> PVFENNNQRYYESLPFKQLKELKIACSQYGPTAPFTIAMIENLGTQALPPNDWKQTARACLSGGDYLLWKSEFFEQCARIADVNRQQGIQTSYEMLIGEGPYQATDTQLNFLPGAYAQISNAARQAWKRL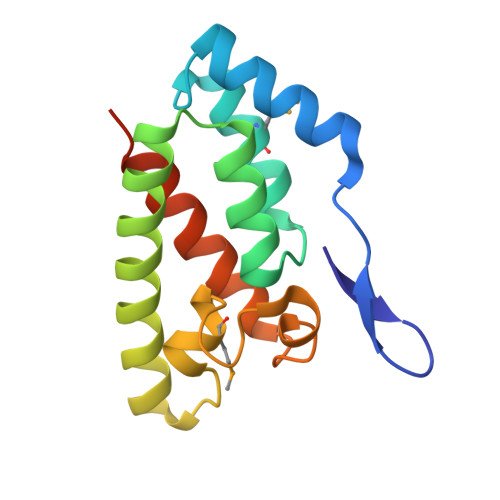PSLEHHHHHH>SNAMDSRFLPATAFIDPEGRNRNEVERLVQQVVDLILAKLTGAAERPPMPETVDLPGPITIPEAAATEATLLQAIRDMVDGSMNPANPGYIGHMDPMPATMAILGDLVAAAVNNNMLSLEMSPSFSRLETLLLRAIAGLFGLGEQAGGVLTSGGSLANLQALAVARNVAFDSVEPGITGLAQRPVIFASEAAHTSLQKAAMLLGLGTAAVIPVRATADSRMDPEDLRARIDQARGAGQHPFCVVATAGTTTTGNIDPLAEIGAIAREHGLW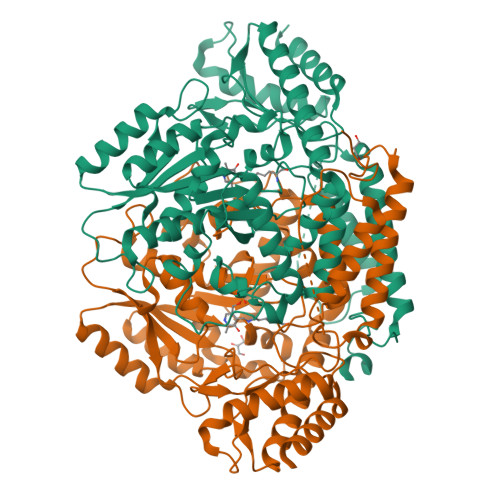FHVDAAYGGALVFSERHRWRLAGIEQADSITFNPQKWLYVAKTCAMVLFRDAGVLERAFRIPAPNMRATDGFINLGEIGVQGTRHADVVKLWLTLQHIGQQGYARLIDDGYRLAERVVEGVRQRPFLRLAGEIDTNIVCFRGEPDWLPAERWDDWNAALQALLLREGKIFLSLPVYRGGRWLRAVLLNPYTTDAVIDAMFKQIDRFAGRERGQER[4x]Here, we report the identification of NADases on the surface of fungi such as the pathogen Aspergillus fumigatus and the saprophyte Neurospora crassa. The enzymes harbour a tuberculosis necrotizing toxin (TNT) domain and are predominately present in pathogenic species. Interestingly, N. crassa NADase (NcNADase) activity was not affected by either EGTA or Ca2+. Both AfNADase and NcNADase cleaved NAD+ and NADP+, but not their reduced counterparts, NADH and NADPH. The absence of ADP-ribosyl cyclase activity from the fungal NADase was further substantiated by its inability to convert the NAD+ analogue nicotinamide hypoxanthine dinucleotide (NHD+) to Nam and fluorescent N7-cyclic inosine diphosphoribose (N7-cIDPR), a reaction specifically observed for cyclases. These results demonstrate that fungal NADases are pure NAD glycohydrolases as they lack both cyclase and base-exchange activity.

To understand the catalytic mechanism of AfNADase and related NADases such as TNT, we attempted to solve the structure of the enzyme in complex with NAD+ by soaking the crystals with the dinucleotide. However, due to the fast conversion rate of NAD+ to Nam and ADPR, it was not possible to trap the substrate in the crystals. We therefore used the non-cleavable NAD+ analogue BAD, differing from NAD+ by the substitution of the nitrogen atom in the pyridine ring with a carbon atom. The structure of the complex clearly illustrates the binding mode of the substrate to the active site, and many of the residues are the same as those involved in product binding. The interaction with BAD includes two water molecules; one is found in the same position as water I in the structure of AfNADase bound to the products and the other, water II, makes contact with the proximal ribose. In the complex, F137 makes contact with the proximal ribose of BAD positioning the scissile bond into the active site. The benzamide (nicotinamide, by analogy) is also held in place by hydrogen bonding to R129, F130 and R148. The sidechain of Q194 makes contact with the 2” OH group of the proximal ribose. We propose a mechanism where water molecule I is hydrogen-bonded to the in-ring oxygen of the proximal ribose, the nicotinamide moiety, the phosphodiester backbone and R129. The nucleophilic attack is further prepared by Q129 which interacts with the 2” OH of the proximal ribose and can potentially induce a δ-negative charge. This mechanism would resemble a SN2 reaction with the formation of a transition state, in which the attack on the α-face on the C1’ position from water II coincides with the nicotinamide leaving and the formation of a partial oxocarbenium ion (oxonium intermediate).

>[2x]MIFTNAILVISALLPATVLSLQHTEDSLFPARCWPDPCAGITFQNDTYVCGDPRLGPVVLPQKFPLNNELRTYARFGALCPAEFLDKWATDVAPNGTYIYPPANGFALDTEEQPILGNATLPVGMKLDRFGSEYGTFLAPLGAPYIERSLPPSNLNTFDGMYPYNYHVYQVTKEFVVGLGPIAPWFEQPGMGTQFVTYTNVLGLIDDGYLRRLDESEYDEKVEYSNPYTPGPNQDVLFQGPGHHHHHH The 9-1-1 DNA checkpoint clamp is loaded onto 5′-recessed DNA to activate the DNA damage checkpoint that arrests the cell cycle. Rad24 replaces Rfc1 and loads the DNA damage 9-1-1 ring onto DNA to signal DNA damage. Unlike RFC, which encircles DNA, Rad24 binds 5′-DNA on its surface, not inside the loader, and threads the 3′ ssDNA overhang into the 9-1-1 clamp from above the ring. Here we describe the first two structures of the Rad24-RFC–9-1-1 clamp bound to DNA and nucleotides, in closed and open conformations, at a resolution of 3.2 Å.

In one conformation the 9-1-1 ring is closed, but in the other the ring is wide open with a 27-Å gap. Here we choose the closed state to illustrate the DNA binding with Rad24 in the loader. The most striking feature is that the DNA is bound only by the Rad24 subunit in an extended groove on its AAA+ module and extending to the collar domain. The third loop is hook-like, projecting from the Rad24 AAA+ domain, and interacts with Ddc1 of the 9-1-1 clamp in the closed state. In the closed conformation, Rad24 sits above Ddc1, having the largest interface of 830 Å2. The interface between Rfc2 and Ddc1 is 400 Å2 in the closed state and is reduced slightly to 350 Å2 in the open state. In both closed and open 9-1-1 clamp states, the first four interfaces (Rad24:Rfc4, Rfc4:Rfc3, Rfc3:Rfc2 and Rfc2:Rfc5) are occupied by ATPγS and Mg2+, and an adenosine diphosphate (ADP) occupies the last interface between Rfc5 and the A′ subdomain of Rad24. Strikingly, the 9-1-1 ring is planar in both the closed and open states of the Rad24-RFC–9-1-1 clamp–DNA complex. The Rad24-RFC complex conformation is essentially unchanged in the 9-1-1–DNA open and closed states.

> MDSTNLNKRPLLQYSLSSLGSQITKWSSSRPTSPVRKARSTENDFLSKQDTSSILPSINDDGGEQWYEKFKPNCLEQVAIHKRKLKDVQEALDAMFLPNAKHRILLLSGPSGCSKSTVIKELSKILVPKYRQNSNGTSFRSTPNEHKVTEFRGDCIVNDLPQMESFSEFLKGARYLVMSNLSLILIEDLPNVFHIDTRRRFQQLILQWLYSSEPLLPPLVICITECEIPENDNNYRKFGIDYTFSAETIMNKEILMHPRLKRIKFNPINSTLLKKHLKFICVQNMKMLKEKNKWNKRQEVIDYIAQETGDIRSAITTLQFWATSSGSLPISTRESTISYFHAIGKVIHGSHSTNNDNEMINNLFENSNNLLSKEDFKLGILENYNTFNKGEFSISDASSIVDCLSECDNMNGLPESNEYGLREVRKTFRNISKQGHNHGTVYFPREWKVRKLQNSFKVQAEDWLNVSLYKYNAVHSFRNITLEFGYYAPLIRKCQSYKKKYILYYLKNLPSGSSGPKQTMDKFSDIMKVENGIDVVDRIGGPIEALSVEDGLAPLMDNDSNNCDHLEDQKKERDRRLRMLIDQYERNVMMANDDLEDEETSFNDDPIVDSDSDNSNNIGNETFGRSDEDESLCEILSQRQPRKAPVISESLSDSDLEIL;> MSKTLSLQLPWVEKYRPQVLSDIVGNKETIDRLQQIAKDGNMPHMIISGMPGIGKTTSVHCLAHELLGRSYADGVLELNASDDRGIDVVRNQIKHFAQKKLHLPPGKHKIVILDEADSMTAGAQQALRRTMELYSNSTRFAFACNQSNKIIEPLQSRCAILRYSKLSDEDVLKRLLQIIKLEDVKYTNDGLEAIIFTAEGDMRQAINNLQSTVAGHGLVNADNVFKIVDSPHPLIVKKMLLASNLEDSIQILRTDLWKKGYSSIDIVTTSFRVTKNLAQVKESVRLEMIKEIGLTHMRILEGVGTYLQLASMLAKIHKLNNKA;> MSTSTEKRSKENLPWVEKYRPETLDEVYGQNEVITTVRKFVDEGKLPHLLFYGPPGTGKTSTIVALAREIYGKNYSNMVLELNASDDRGIDVVRNQIKDFASTRQIFSKGFKLIILDEADAMTNAAQNALRRVIERYTKNTRFCVLANYAHKLTPALLSRCTRFRFQPLPQEAIERRIANVLVHEKLKLSPNAEKALIELSNGDMRRVLNVLQSCKATLDNPDEDEISDDVIYECCGAPRPSDLKAVLKSILEDDWGTAHYTLNKVRSAKGLALIDLIEGIVKILEDYELQNEETRVHLLTKLADIEYSISKGGNDQIQGSAVIGAIKASFENETVKANV;> MFEGFGPNKKRKISKLAAEQSLAQQPWVEKYRPKNLDEVTAQDHAVTVLKKTLKSANLPHMLFYGPPGTGKTSTILALTKELYGPDLMKSRILELNASDERGISIVREKVKNFARLTVSKPSKHDLENYPCPPYKIIILDEADSMTADAQSALRRTMETYSGVTRFCLICNYVTRIIDPLASRCSKFRFKALDASNAIDRLRFISEQENVKCDDGVLERILDISAGDLRRGITLLQSASKGAQYLGDGKNITSTQVEELAGVVPHDILIEIVEKVKSGDFDEIKKYVNTFMKSGWSAASVVNQLHEYYITNDNFDTNFKNQISWLLFTTDSRLNNGTNEHIQLLNLLVKISQL;> MSLWVDKYRPKSLNALSHNEELTNFLKSLSDQPRDLPHLLLYGPNGTGKKTRCMALLESIFGPGVYRLKIDVRQFVTASNRKLELNVVSSPYHLEITPSDMGNNDRIVIQELLKEVAQMEQVDFQDSKDGLAHRYKCVIINEANSLTKDAQAALRRTMEKYSKNIRLIMVCDSMSPIIAPIKSRCLLIRCPAPSDSEISTILSDVVTNERIQLETKDILKRIAQASNGNLRVSLLMLESMALNNELALKSSSPIIKPDWIIVIHKLTRKIVKERSVNSLIECRAVLYDLLAHCIPANIILKELTFSLLDVETLNTTNKSSIIEYSSVFDERLSLGNKAIFHLEGFIAKVMCCLD;> MKLKLIVNGCEAPDDYKLLRTTINTVASLRKTAILRFNSERLTIISTPKSSLNSSNNGTILRGDTGQLWCTIPHDVFRLYTVISARELNTITMECNCDSLLSVFKRYDRVMNQGSSSNMTIKLQSMPEWNTNNGTLSGGTAGGVDTTSKPNPICALGITFEEIVHTSGPNDAIVMNGGVDEHNGLPTTVGTGNLLASNKVIMHSFKVPVKLLFRAQDTRIQEPMINYIQLMMYKLPPISGEFGSAFHGFIRRVERYSNVNHIHLMGVKKKEHGNEGDDVELKIIVNELDWHLEICWNGPLDSVIQRQEGLTDNPSQNQHIDTDGRQEEGSLPIIEADKPMSSLYTNTRDREMEENIRYDEDLLRIEDSSIADTRGNIYTADTSGDTEFNDISVMVEKAEQESSSTHEVIIRCKDWKVCSKLYAAFEEVVLAISHDESCVFHCSLDERGQIIYYIARSKGL;> MRINSELANKFSASTVHLEHITTALSCLTPFGSKDDVLIFIDADGLSFVRENNHVIKIQLLLSRELFMSYSYRNETEDHMKLCVKINHILDSVSVMNRNSDDIVECTLSYDGHGSPFVLIFEDSFISERVEYSTYLIKDFDTNGLELDRERISFEAIIKGEALHSALKDLKEIGCKECYVYAKTEANDENVFALISKSQLGFSKIKLPSNRSILEKLQVFDGDSTTVIDGFAVIGFFDFTSFDKIRKSTKIASKVLFRMDVHGVLSVNILSQTDDVIITDTTRPSNNRPGSIRQLQLPKDYPGIVIEVCMLEKESIDEAAQTEIELLMETNELGNRNSFKKSTIRKRYGTDKGNETSNDNLLQLNGKKIKLPSEEENNKNRESEDEENHCKYPTKDIPIFF;> MSFKATITESGKQNIWFRAIYVLSTIQDDIKITVTTNELIAWSMNETDTTLCQVRFQKSFFEEYEFKPHEIVFGENGVQVIEDTYGNSHKLYSFRVNGRHLTTISRKPDGDGIKSFTIAVNNTSTCPESLANRLIVVIEMDSLIVKEYCPQFQPIKYDPIIINLKYKRRFLDVFGTAASDRNPQEPLDPKLLDVFTNTERELTSALFNEEVESDIRKRNQLTAADEINYICCNSTLLKNFLDNCNVNVTDEVKLEINVHRLSITAFTKAVYGKNNDLLRNALSMSNTISTLDLEHYCLFTKSIIFKLKDFKNFITIGPSWKTTQDGNDNISLWFCHPGDPILMQMQKPGVKLELVEVTDSNINDDILEGKFIKTAISGSKEEAGLKDNKESCESPLKSKTALKRENLPHSVAGTRNSPLKVSYLTPDNGSTVAKTYRNNTARKLFVEEQSQSTNYEQDKRFRQASSVHMNMNREQSFDIGTTHEVACPRNESNSLKRSIADICNETEDPTQQSTFAKRADTTVTWGKALPAADDEVSCSNIDRKGMLKKEKLKHMQGLLNSQNDTSNHKKQDNKEMEDGLGLTQVEKPRGIFD> GSVHKHTGRNCGRKFKIGEPLYRCHECGCDDTCVLCIHCFNPKDHVNHHVCTDICTEFTSGICDC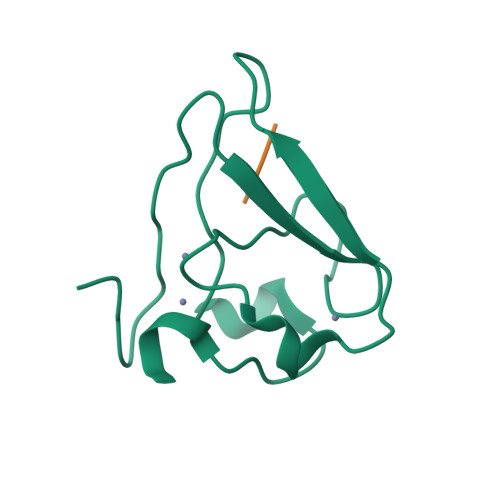GDEEAWNSPLHCKAEEQ;> HIAA1,1,5,5-TETRAFLUOROPHOSPHOPENTYLPHOSPHONIC ACID ADENYLATE ESTER | 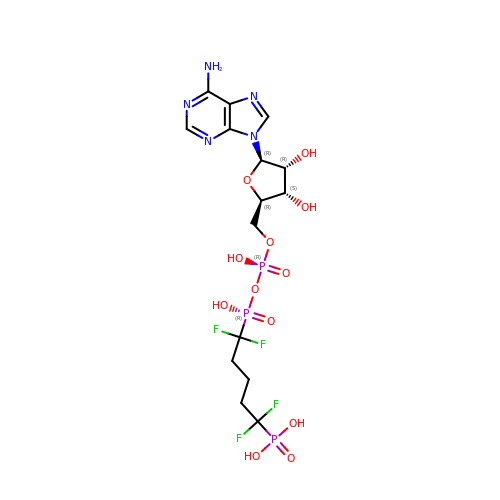C15 H22 F4 N5 O12 P3 | VWQBAZQMKBHYJA-QYVSTXNMSA-N> TGEVKRPETSAPVPPLIKEATYIEATASGYMAEGVLNPTIILRRGQRVDMTLKNKLTEPTIVHWHGFDVNWHNDAHPSFAITPGESYNYSFDVVNRAGTYLYHPHPHGLTAKQFYMGQLGLVIVEDSGSDLGFKYGVNDLPLV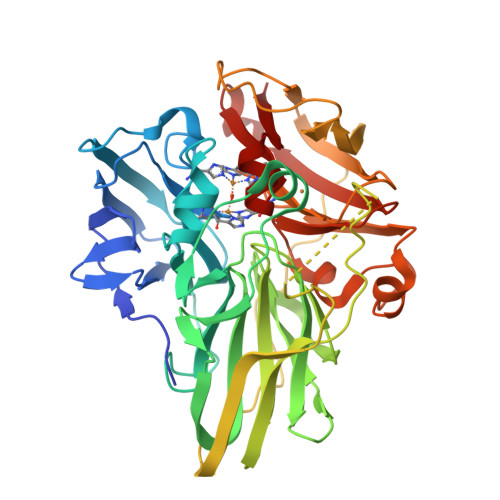ISDRRFIGGAPVYNPTPMEMIAGFLGNAVLVNGVKDAVFKLSGGSYRLRLVNGSNARLYMLSIVKKNGDVVPMRLIAVDQGFLARPIEVRALFLAPAERAEVVVELGEGVYLLKNTPIDPMHLEMGHGMQEALPEGSEYTIATFLVEGKGEAVPVEALSDPPPEPPKPTRTRRFALSLSGMQWTINGMFWNASNPLFEHVSVEGVELWEIVNDKASMPHPMHLHGFPMWIIERKDSPRQVAELAVDNRGRLPTDLGLKDTVLIWPGETVKIVVNFDAKKRGQLFPFHCHNLEHEDGGMMINIAVK>SQDASDGLQRLHMLQISYFRDPYHVWYQGNASLGGHLTHVLEGPDTNTTIIQLQPLQEPESWARTQSGLQSYLLQFHGLVRLVHQERTLAFPLTIRCFLGCELPPEGSRAHVFFEVAVNGSSFVSFRPERALWQADTQVTSGVVTFTLQQLNAYNRTRYELREFLEDTCVQYVQKHISAENTKGSQTSRSYTS[4x]

EPCR is a transmembrane MHC class I-like glycoprotein primarily abundant in the vasculature of large vessels, but present in numerous cell types. Since its identification, EPCR has been mainly known for its role in accelerating the generation of the anticoagulant activated protein C (APC) and favoring its cytoprotective properties. Structurally, EPCR shares a notable degree of homology with the CD1 family of receptors, including the presence of a central and extended hydrophobic cavity suitable for lipid antigens, flanked by two alpha helices lying on top of a beta sheet. The presence of a lipid bound to EPCR is key for its biological functions.

For this, we performed a wide crystallization screen and obtained EPCR crystals in varied conditions, which ultimately led to solution of the structure in three different space groups. Crystals grown in other conditions yielded EPCR structures in two novel space groups, C2221 and P212121, containing 2 and 4 molecules of EPCR per asymmetric unit, respectively. Structural alignment against EPCR in space group P3121 yielded root mean square deviations of 0.459 and 0.400 for EPCR molecules in space groups C2221 and P212121. EPCR in P3121 and P212121 space groups present strong and continuous Fobs-Fcalc difference maps that suggest a prevalent diacyl molecule but a more ambiguous head group moiety. Fitting of a diacyl phospholipid scaffold (lacking the outermost head group) satisfied the overall shape of the map, albeit with some degree of uncertainty for the orientation of the carbonyl groups. In order to assess the later, we mapped the atomic displacement parameters (ADPs, also known as B-factors) in all space groups in which EPCR was crystallized. The P3121 space group yield the highest B-factors for all atoms, while those EPCR-lipid complexes present in the P212121 crystal structure showed the most rigid atom positions, as suggested by the lower B-factor values. Amongst all EPCR molecules in the three space groups obtained, the dimensions of the pockets range from ~ 1280 to ~ 1615 Å3, where both values were found in two of the four EPCR molecules present in the P212121 space group asymmetric unit.> MSSVLKAFERFTIEQELQDRGEEGSIPPETLKSAVKVFVINTPNPTTRYQMLNFCLRIICSQNARASHRVGALITLFSLPSAGMQNHIRLADRSPEAQIERCEIDGFEPGTYRLIPNARANLT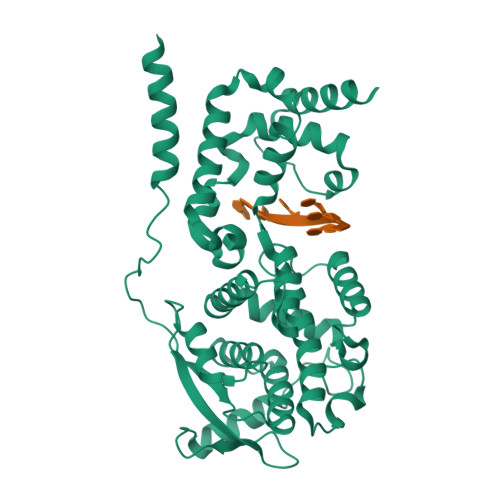ANEIAAYALLADDLPPTINNGTPYVHADVEGQPCDEIEQFLDRCYSVLIQAWVMVCKCMTAYDQPAGSADRRFAKYQQQGRLEARYMLQPEAQRLIQTAIRKSLVVRQYLTFELQLARRQGLLSNRYYAMVGDIGKYIENSGLTAFFLTLKYALGTKWSPLSLAAFTGELTKLRSLMMLYRGLGEQARYLALLEAPQIMDFAPGGYPLIFSYAMGVGTVLDVQMRNYTYARPFLNGYYFQIGVETARRQQGTVDNRVADDLGLTPEQRTEVTQLVDRLARGRGAGIPGGPVNPFVPPVQQQQPAAVYEDIPALEESDDDGDEDGGAGFQNGVQLPAVRQGGQTDFRAQPLQDPIQAQLFMPLYPQVSNMPNNQNHQINRIGGLEHQDLLRYNENGDSQQDARGEHVNTFPNNPNQNAQLQVGDWDE>MLYEEDYKLALEAFKKVFNALTHYGAKQAFRSRARDLVEEIYNSGFIPTFFYIISKAELNSDSLDSLISLFSSDNAILRGSDENVSYSAYLFIILYYLIKRGIIEQKFLIQALRCEKTRLDLIDKLYNLAPIISAKIRTYLLAIKRLSEALIEAR[3x];>MPYYAFAEPFFIHAITHLHVGSGSSVEEEIALPFQRDELGYPTIYASSLKGAIKSFLLKEFPDKRDVIYKVLGEDENPEEASLGTFLDAILFAIPSRIIEIDSAKPYVWVYVTTYELLKKVKLYLDSISQLSNASFSNLKNKIDTILAKEGKNITLDSDLKSAILNEDFYVELEALNNKIPSIINAGVPLLVLEDSIGREVINRSLIRVRRIRIDRDKKVVETGGLWSEEYVPMKTIFFSVLLGKESKESAIFASCILRNLRYVILGGKETIGKGIVELRWVKDVI[4x];> MKRVLIKPLEPLMFRSQGEFEPLITGSHTAAQSLIIPRPSTIAGMLGYILFNKSSGTGDWLSDLTNLLATIYGTFIETNGEYLFPLRMGNHLALVDQQHLINLPTLLEKEYERREKGIYELFYDKNKLFQIINHQDRIGISIDKSTRTVKEHYLYSARYLAFKKEVNYVIFIDNDAISDKINGKIVNFGGENRIAKLEVDDYKVDTSIEEEYYLALSPILIPDEALDNFLDNISDYVAMGKVDKISLGFDIANTKRKEMLTAILEGSIVKRSIIDFIKNEIKNDLRYRFSKYEKIGYNTLMSLCKLALRKILS;> MAIDFLVNILELIKEKQCNINLFSAISLTSIVYNNFGEFLSNNQSYSTNNPLLKYHIIILNDKNKTKDVEEKRNIFKREVAELISRNFKLDGEKVRNYFDSLKEVLKSLKYTIVDVEITTRTRALIGVSTSLGKLIFGSGISFDPYMNLPYIPASEIKGIVRSYIEGKLGEQEAEEIFGNEEREGNVNFTDAYPTRSKDFLFVPDVITPHYNGKKSEADAEPRPVIHLTIAPKVTFRFLIYYKREDVGKPICDSMPIILIRGLGARSSVGYSLFELRKIEVIKAAAHHHHHHHHHH;> MEELLMSLKLKALYPLTGGYNRHSINPFYEELVRPTEIKGLWRWWNRVLFNTLAYSTKGKLYTYESIDRLFEDVFGSENKKSAVRLEVITDEGNDNRFELSYVELDKVIDCLRNYKRKVSLDFIDNTLIAEIEGSTKIPISFKSNLDIDKIIKDLVHNNKLLSFELLGFKSVEIDATKISDKKILKEILRDLITNYLEYFNIKQEVTFTLNIYLDKSREHKQNFEDKLKFALYSLLVFILLGGIGRKTSRGFGSLSIIDVKCYDNSICKKIEDLAKNFLKISSGNELKSKIESILDCIKNSCIDTLYIENNILSEIDPKKNVVYFINSDLFEVKRINDKEKVLANIYKAVSSEGCCIKSIITDKYVRKSFLIAFGGYRKVEKDKGLDIGFIKNYLCETCETVSSFNIVDFLLSEGSFMSDYILQYEHRNSLLRFKLISDNSNNSYLIGYILHSSYFKKIDIKYVRCILEKLTYCVI;> MSIDNVLREFLDYKIIALLHDPPNKAWVITGRARNLTQQLSNIRASRKHEKVAKYIINQLFGKNYSEKVDNADKLASSIDRYLGSIVYKERSLFENRSIFLKNILLSNIQRDIGNLFPKDKSKLDNLILEYKKLLNVINKTNLILKYQLFYLIYELVWIDSKYENTPSDTRNPTHTIFDHLYATAAMMNWILSLEKEAKGYLLGIDTIGVADFISKGRKTRDLWISSYLVSALLWYVITWFIEEYGPDVILFPSLRFNQFYAFYLLEKLRKEGVSEDVIDEIKELITKYIFNGDDLFENLKIPPYPIIPGRITLILPGLIREGEEYKKVQDDNCFISKVKERYNEGWRKLIEGLRCYSERKREDGFWNLVCRVLKLTEDLLQTTPLNIRVKQVSVTEDEIFNNNKLRSDSWKIYDNKYRQLVSEFKKSKLVKVTPESRLKLFELTKFDKLPQIGEKSKRGYEFCTSCGVLPAVVIMPKEDELEKKLIDLGIARDEKDVRSIKNMISPGERLCPWCLVKRALGAEPRLMRILLLGDLYSVEKIVNEIVSRDVKIEIPSTSDIASIKTFEEMIEKKNEICEDLKEEEVCEKPSESVLSMWQWFNKNYYNGINLTIDPEEYWFSEKRRRYYFSVFRRHRITFPSPYYALVRADSDYLGDLLEGKLTPYLAGIIDSGDYANISEKKEEVNKLLEEYLVNAGSGSIVDYVKTVLKCIRENLNKCSCAEKIYSNEVAKVMFRVNVEKANVEEEVKNSLEYFETILNEGRIIVTPAWHVSISSALNRGLLVELELVNKHKGFVIYAGGDDLLAMLPVDEVLDFIKESRRAFAGFGTEKLGNMCLENGFVRINNAYYPSLPIVGRSYSVIIAHYADPLFFVINDSYNLLEEGKEIIRYRVMYNGEYKDAKKDVAIFRYQGLTSVIPLSLKRPIVSSVSDFNEIASIIDVILELKKRIDEGRISVSLLYDYEKYKHLIVASDEKYLTEFLVKDWIKRNSLRKHVEFTIDEKLYGVRLTIENYPIKIPNDLISNIVYTLRIIYGGEK;>[22x]MSTQREYVFIPITNSITIDVKITIGGSDHITNIDERGIHNVLVITGYAVDEKNGRL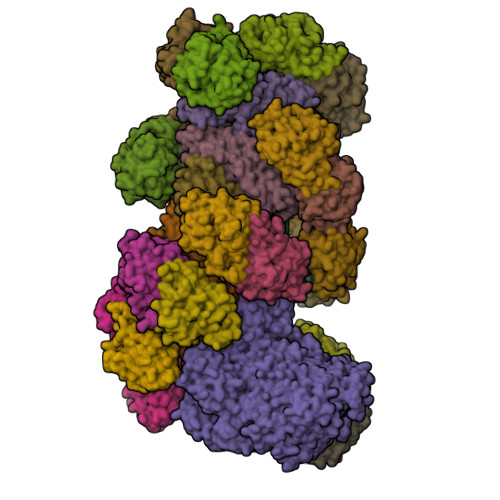VPTLDPCDYVKGILVAGTPQQAQSNDFLTLKLPANKLYLIRKKGNISDDLKIYIPYSSPDARNSMKTKPVSISDDTIVNNIIKEVFDKIYNITQKEKVKIEKVKEDIKELFSYYALEQ> MEHHKTYHSANIKTATGSLLIEGPVSPEDLAGYEFHKDLTAFRPPREQHEALVDIAGLPEGRII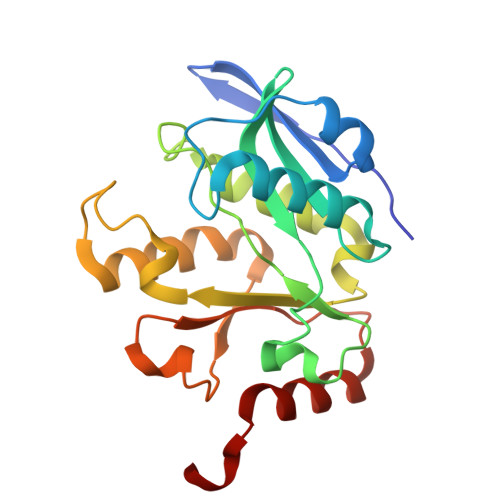IARDGRTIVGYVTYLYPDPLERWSEGNMEDLIELGAIEVAPDYRGCAVGKTLLTVSMMDEQMENYIVMTTEYYWHWDLKGMKKDVWEYRKIMEKMMNAGGLVWFATDEPEISSHPANCLMARIGKNVSQESIEQFDRLRFYHRYMY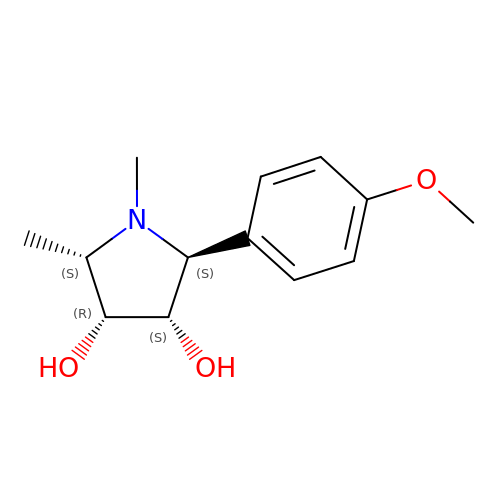(2S,3S,4R,5S)-2-(4-methoxyphenyl)-1,5-dimethylpyrrolidine-3,4-diol | C13 H19 N O3 | GJZNAEFHIYPPEM-KNDHEWATSA-N>MDTNPCEKHSCIAVIDAGSTGSRLHIYSYDTDDTNTPIHIEEIWNKKIKPGFASIQPNSVTIDAYLTMLLADAPIHNIPVYFYATAGMRLLPQSQQKKYYDELDYWFRQQSQWQLVEAKTITGNDEALFDWLAVNYKLDTLKSVQNKSVGVMDMGGASVQIVFPMPKNAEISKHNQVELNIYGQNINLYVHSFLGLGQTEMSHQFLNSPSCFANDYPLPDGESGQGNAPSCKEEVTSLMNSVHKVNQQIQPLLALNPVNEWYSIGGISNLASSQLFHFENSELTNQS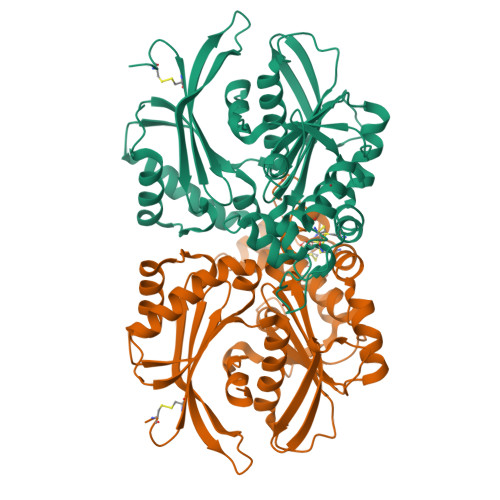LLQQGDNQICHQQWDILNGQYPDDEYLYQYCLLSSYYYALMVDGYGINPNQTIHYIPPEQNLDWTIGVVLHRALEHHHHHH[4x]>[6x]ELDKWASLWNWFNITNWLWYI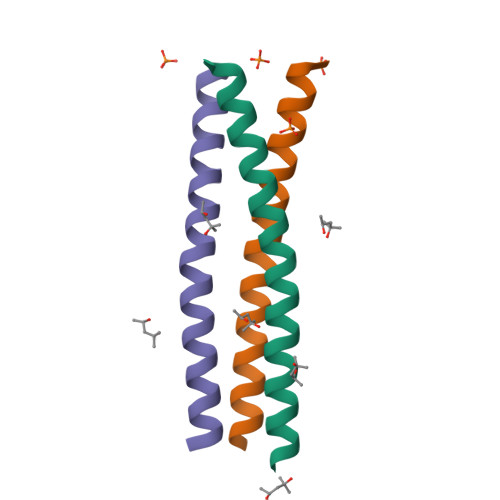KIEELKSKIKRIENEIKRIKK>[2x]GSHMASTISVKDENGTVKVPKDAKRIVVLEYSFADALAALDVKPVGIADDGKKKRIIKPVREKIGD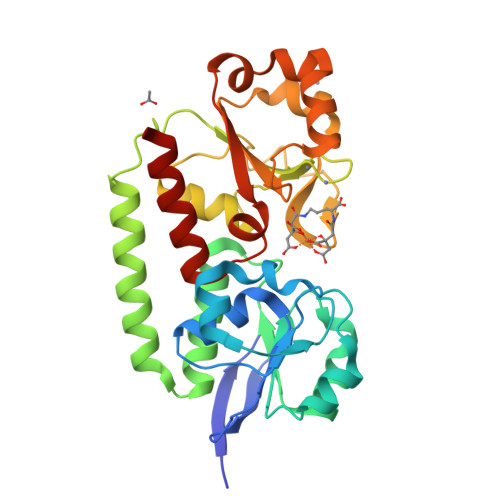YTSVGTRKQPNLEEISKLKPDLIIADSSRHKGINKELNKIAPTLSLKSFDGDYKQNINSFKTIAKALNKEKEGEKRLAEHDKLINKYKDEIKFDRNQKVLPAVVAKAGLLAHPNYSYVGQFLNELGFKNALSDDVTKGLSKYLKGPYLQLDTEHLADLNPERMIIMTDHAKKDSAEFKKLQEDATWKKLNAVKNNRVDIVDRDVWARSRGLISSEEMAKELVELSKKEQK> MSEVKPMSHVKEVDVEEEKLFFDENQPEMVEGEEETVSSASAPEVLAKMCVAVEAIHQLSDIYAITKLEGVSKPDVDGIRALVKRMSTEGFEAPKKAVASLEQYASMFTPTRSTLNVTISQEAVMATIINTLKTWFEKLMELFAKLIRWISDFKKRDVVVATRYGKIVRAVDQARTLFQELLVKNRLGNRKDALLEKFDAIAQSIIDDPKILASRIYAAAFGSVY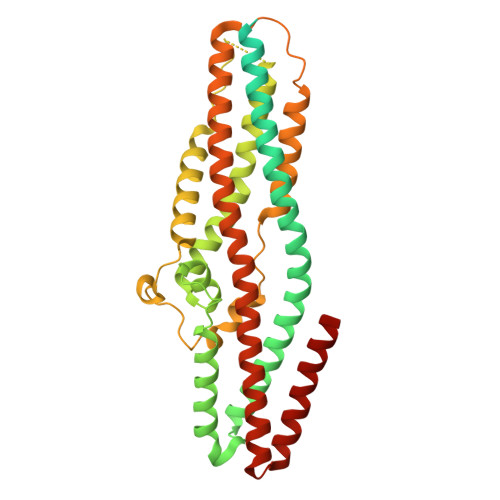YQKEIININNEARTELGTMEKLVGTIIEYVNYNGDDYRALMPIANIREIGKLATRCNELSTVYPDRSSIPDFPDKNFWKNSHLLKDRFVAPLDDLLKAYRNSSDALRKLKQLSRNYSQETIDAIGESVQLINTSLEGMRRITDTMFEYSQAQYLAASCVLNYYGKCAQVVSEDYKIHGFNDAIREWQRRFDKVIDDFKRGYAM> PHMSGLKKFFPYSTNVLKGAAADIALPSLAGKTVFFYFSAS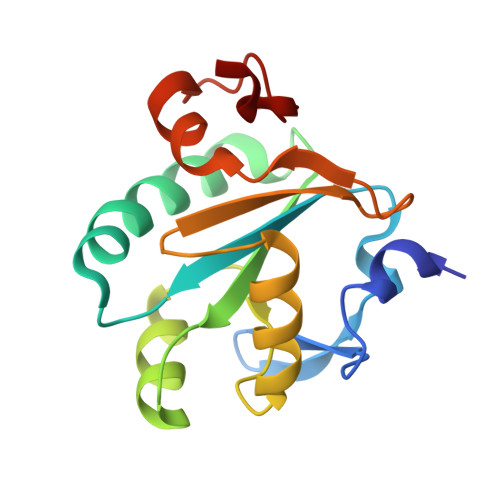WCPPCRAFTPQLIDFYKAHAESKNFEVMLISWDESAEDFKDYYAKMPWLALPFEDRKGMEFLTTGFDVKSIPTLVGVEADSGNIITTQARTMVVKDPEAKDFPWPNVEAKK CDT is a member of the Iota family of protein toxins which also consists of two homologous toxins produced by Clostridium perfringens (the Iota toxin) and Clostridium spiroforme (C. spiroforme Transferase, CST). All three Iota toxin family members are assembled from two polypeptide chains termed the “A” subunit (CDTa, Ia, and CSTa) and “B”, subunit (CDTb, Ib, and CSTb). All three B subunits are presumed to contain five domains that are involved in regulation (D1), oligomerization (D2 and D3), and host recognition (D3’ and D4). Once proteolyzed, the mature form of CDTb forms a large heptameric, soluble structure referred to as the prepore which binds one molecule of CDTa to generate the toxic moiety, CDT.

However, due to significantly lower particle counts for the larger oligomeric intermediates, a decrease in resolution was observed for all intermediate structures containing more than three protomers. A map of the tetrameric intermediate was refined after rebalancing particles to limit issues arising from preferred orientation leading to a map of 7.01 Å resolution. The helical nature of the oligomeric intermediates is also observed in the model of the tetrameric intermediate which illustrates a separation of ~46 Å across the tetramer. When propagated about the asymmetric heptameric structure, this would account for a total separation of ~15 Å in the vertical dimension and ~58 Å in the horizontal direction forming a ‘lock-washer’ like structure and indicating the structural plasticity observed across the oligomerization interface is not restricted to two-dimensional space.

>[4x]MKIQMRNKKVLSFLTLTAIVSQALVYPVYAQTSTSNHSNKKKEIVNEDILPNNGLMGYYFTDEHFKDLKLMAPIKDGNLKFEEKKVDKLLDKDKSDVKSIRWTGRIIPSKDGEYTLSTDRDDVLMQVNTESTISNTLKVNMKKGKEYKVRIELQDKNLGSIDNLSSPNLYWELDGMKKIIPEENLFLRDYSNIEKDDPFIPNNNFFDPKLMSDWEDEDLDTDNDNIPDSYERNGYTIKDLIAVKWEDSFAEQGYKKYVSNYLESNTAGDPYTDYEKASGSFDKAIKTEARDPLVAAYPIVGVGMEKLIISTNEHASTDQGKTVSRATTNSKTESNTAGVSVNVGYQNGFTANVTTNYSHTTDNSTAVQDSNGESWNTGLSINKGESAYINANVRYYNTGTAPMYKVTPTTNLVLDGDTLSTIKAQENQIGNNLSPGDTYPKKGLSPLALNTMDQFSSRLIPINYDQLKKLDAGKQIKLETTQVSGNFGTKNSSGQIVTEGNSWSDYISQIDSISASIILDTENESYERRVTAKNLQDPEDKTPELTIGEAIEKAFGATKKDGLLYFNDIPIDESCVELIFDDNTANKIKDSLKTLSDKKIYNVKLERGMNILIKTPTYFTNFDDYNNYPSTWSNVNTTNQDGLQGSANKLNGETKIKIPMSELKPYKRYVFSGYSKDPLTSNSIIVKIKAKEEKTDYLVPEQGYTKFSYEFETTEKDSSNIEITLIGSGTTYLDNLSITELNSTPEILDEPEVKIPTDQEIMDAHKIYFADLNFNPSTGNTYINGMYFAPTQTNKEALDYIQKYRVEATLQYSGFKDIGTKDKEMRNYLGDPNQPKTNYVNLRSYFTGGENIMTYKKLRIYAITPDDRELLVLSVD> MEMDYKDDDDKGGGGGASTMSGTKPDILWAPHHVDRFVVCDSELSLYHVESTVNSELKAGSLRLSEDSAATLLSINSDTPYMKCVAWYLNYDPECLLAVGQANGRVVLTSLGQDHNSKFKDLIGKEFVPKHARQCNTLAWNPLDSNWLAAGLDKHRADFSVLIWDICSKYTPDIVPMEKVKLSAGETETTLLVTKPLYELGQNDACLSLCWLPRDQKLLLAGMHRNLAIFDLRNTSQKMFVNTKAVQGVTVDPYFHDRVASFYEGQVAIWDLRKFEKPVLTLTEQPKPLTKVAWCPTRTGLLATLTRDSNIIRLYDMQHTPTPIGDETEPTIIERSVQPCDNYIASFAWHPTSQNRMIVVTPNRTMSDFTVFERISLAWSPITSLMWACGRHLYECTEEENDNSLEKDIATKMRLRALSRYGLDTEQVWRNHILAGNEDPQLKSLWYTLHFMKQYTEDMDQKSPGNKGSLVYAGIKSIVKSSLGMVESSRHNWSGL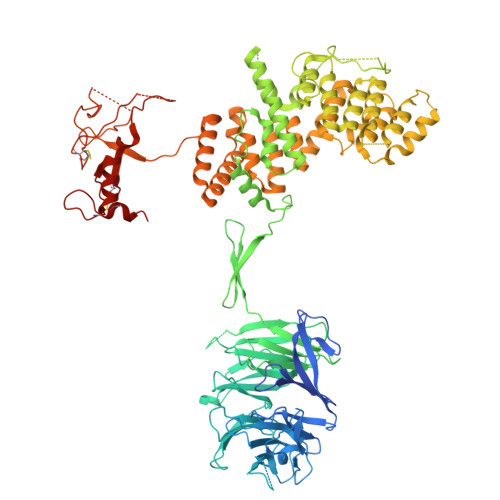DKQSDIQNLNEERILALQLCGWIKKGTDVDVGPFLNSLVQEGEWERAAAVALFNLDIRRAIQILNEGASSEKGDLNLNVVAMALSGYTDEKNSLWREMCSTLRLQLNNPYLCVMFAFLTSETGSYDGVLYENKVAVRDRVAFACKFLSDTQLNRYIEKLTNEMKEAGNLEGILLTGLTKDGVDLMESYVDRTGDVQTASYCMLQGSPLDVLKDERVQYWIENYRNLLDAWRFWHKRAEFDIHRSKLDPSSKPLAQVFVSCNFCGKSISYSCSAVPHQGRGFSQYGVSGSPTKSKVTSCPGCRKPLPRCALCLINMGTPVSSCPGGTKSDEKVDLSKDKKLAQFNNWFTWCHNCRHGGHAGHMLSWFRDHAECPVSACTCKCMQLDTTGNLVPAETVQP> MENDPNLFVALYDFVASGDNTLSITKGEKLRVLGYNHN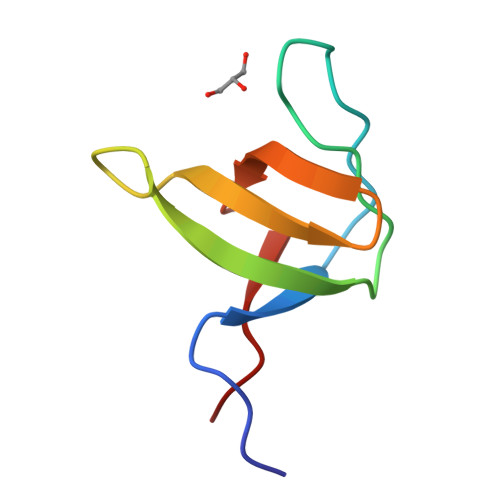GEWCEAQTKNGQGWVPSQYITPVNS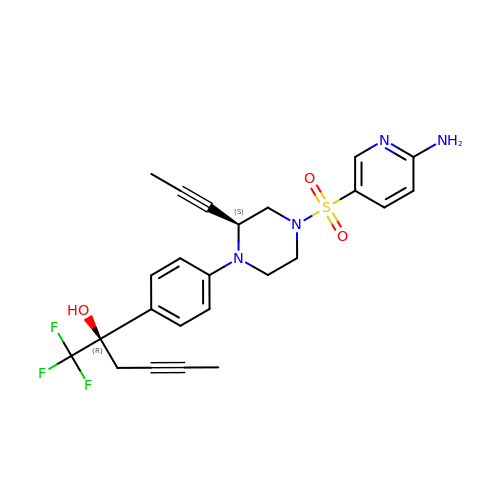(2R)-2-{4-[(2S)-4-[(6-aminopyridin-3-yl)sulfonyl]-2-(prop-1-yn-1-yl)piperazin-1-yl]phenyl}-1,1,1-trifluorohex-4-yn-2-ol | C24 H25 F3 N4 O3 S | DWZSLEBNXFXVGP-NZQKXSOJSA-N3-AMINO-6-{4-CHLORO-3-[(2,3-DIFLUOROPHENYL)SULFAMOYL]PHENYL}-N-METHYLPYRAZINE-2-CARBOXAMIDE | C18 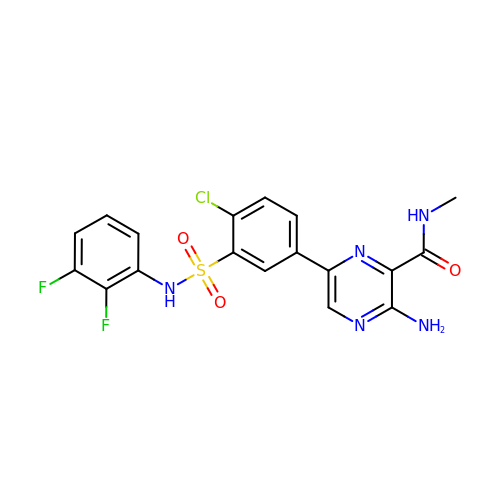H14 Cl F2 N5 O3 S | GEYLKEHPEKRUTC-UHFFFAOYSA-N Sclerotium rolfsii lectin (SRL) is a cell wall-associated developmental–stage specific lectin secreted from the soil–born pathogenic fungus. SRL displays a clear specificity for TF and its substituted glycan structures. In the current study we report two recombinant variants SSR1 and SSR2, generated by the deliberate changes of the amino acids incorporated at particular sites of SRL by the synthetic gene construct method based on the complete amino acid sequence of SRL. Interestingly, SSR1 and SSR2 the two different variants of SRL, differ in their glycan specificity.

Apart from the carbohydrate binding site residues other deliberate replacement of the amino acid is incorporated between SRL and SSR1 at 14th, 113th and 123rd positions, where the amino acids Asn, Glu and Glu residues were replaced by Asp, Gln and Gln, respectively. The crystal structures of SSR1 and SSR2 lectins in their free form were determined at 1.7 Å and 1.6 Å resolution, respectively. Like SRL there are two protein molecules (named mol A and mol B) in the crystallographic asymmetric unit of both variants related by a non-crystallographic two-fold symmetry. The mutations of SSR1 (N14D, E113Q, E123Q) and SSR2 (T1V, N14D, T34S, E113Q, E123Q) were all identified and all atoms of the mutated residues were well defined within the electron density map. Overall the crystal structures of SSR1 and SSR2 are similar to the SRL structure and the introduction of the mutations did not seem to affect the overall structure of the protein. Only, the mutation N14D seems to cause a minor disturbance in the loop region of residues 12–14 in both variants (rms displacement of all atoms 0.18 Å and 0.26 Å from the SRL structure, respectively). The most profound conformational difference is on SSR1 and especially on the side chain of Asn81 which moves away by 5 Å from its position in the SRL structure towards the secondary carbohydrate binding site. The adoption of this conformation of Asn81 in SSR1 is made possible by a shift of the entire loop encompassing residues 81–86 by 3.0 Å on average, from their positions in the SRL structure. The glycan array analysis of the variants demonstrated that SSR1 recognizes TF antigen and its derivatives with high affinity like SRL but showed the highest affinity towards the sialylated Tn antigen, unlike SRL.

>[2x]TYKITVRVYQTNPDAFFHPVEKTVWKYANGGTWTITDDQHVLTMGGSGTSGTLRFHADNGESFTATFGVHNYKRWCDIVTNLAADETGMVINQQYYSQKNREEARERQLSNYQVKNAKGRNFQIVYTEAEGNDLHANLIIG>MELLFLGTGAGIPAKARNVTSVALKLLEERRSVWLFDCGEATQHQMLHTTIKPRKIEKIFITHMHGDHVYGLPGLLGSRSFQGGEDELTVYGPKGIKAFIETSLAVTKTHLTYPLAIQEIEEGIVFEDDQFIVTAVSVIHGVEAFGYRVQEKDVPGSLKADVLKEMNIPPGPVYQKIKKGETVTLEDGRIINGNDFLEPPKKGRSVVFSGDTRVSDKLKELARDCDVMVHEATFAKEDRKLAYDYYHSTTEQAAVTAKEARAKQLILTHISARYQGDASLELQK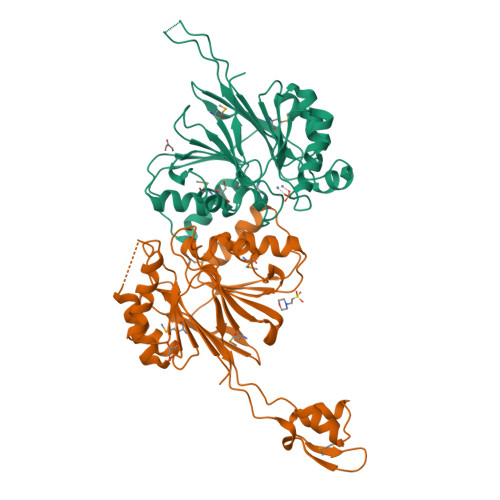EAVDVFPNSVAAYDFLEVNVPRGKLAAALEHHHHHH[2x]> MAYPDANLLNDRVLRAMLKAEETCAPSVSYFKCVQKEVLPSMRKIVATWMLEVCEEQ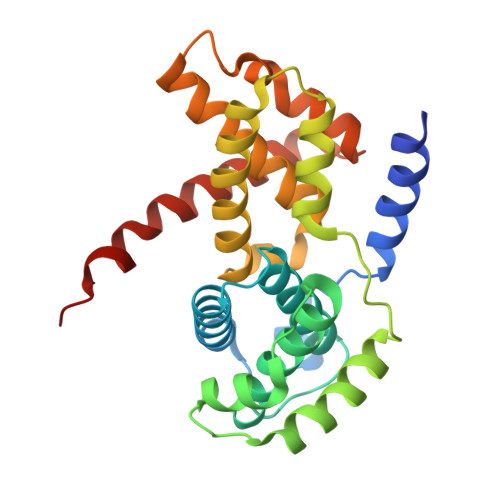KCEEEVFPLAMNYLDRFLSLEPVKKSRLQLLGATCMFVASKMKETIPLTAEKLCIYTDNSIRPEELLQMELLLVNKLKWNLAAMTPHDFIEHFLSKMPEAEENKQIIRKHAQTFVALCATDVKFISNPPSMVAAGSVVAAVQGLNLRSPNNFLSYYRLTRFLSRVIKCDPDCLRACQEQIEALLESSLRQAQQNMDPKAA> MAKKDEVGGRVLQDVFLDWAKKYGPVVRVNVFHKTSVIVTSPESVKKFLMSTKYNKDSKMYRALQTVFGERLFGQGLVSECNYERWHKQRRVIDLAFSRSSLVSLMETFNEKAEQLVEILEAKADGQTPVSMQDMLTYTAMDILAKAAFGMETSMLLGAQKPLSQAVKLMLEGITASRNTLAKFLPGKRKQLREVRESIR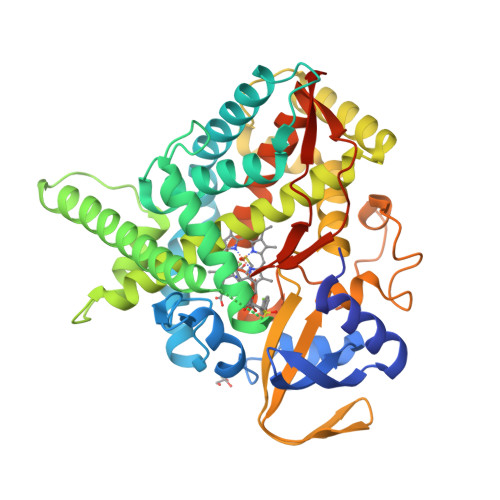FLRQVGRDWVQRRREALKRGEEVPADILTQILKAEEGAQDDEGLLDNFVTFFIAGHETSANHLAFTVMELSRQPEIVARLQAEVDEVIGSKRYLDFEDLGRLQYLSQVLKESLRLYPPAWGTFRLLEEETLIDGVRVPGNTPLLFSTYVMGRMDTYFEDPLTFNPDRFGPGAPKPRFTYFPFSLGHRSCIGQQFAQMEVKVVMAKLLQRLEFRLVPGQRFGLQEQATLKPLDPVLCTLRPRGWQPAPPPPPCHHHH>MSLGQQQVTLFWSGAITGPTSDAGAPYGAAVEDYCKWANERKLVPGVVFNCVVRDDQYNNANTQRFFEEAVDRFKIPVFLSYATGANLQLKPLIQELRIPTIPASMHIELIDPPNNDYIFLPTTSYSEQVVALLEYIAREKKGAKVALVVHPSPFGRAPVEDARKAARELGLQIVDVQEVGSGNLDNTALLKRFEQAGVEYVVHQNVAGPVANILKDAKRLGLKMRHLGAHYTGGPDLIALAGDAAEGFLWATSFYMAHEDTPGIRLQKEIGRKYGRPENFIESVNYTNGMLAAAIAVEAIRRAQERFKRITNETVYQAIVGMNGPNAFKPGFAVSTKQGVEIDFTKSEHTGA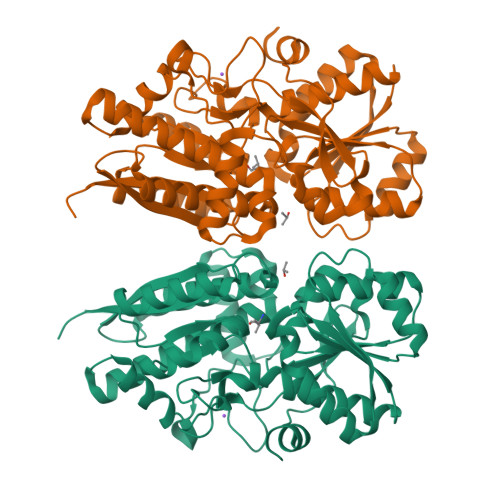EGLRILEAKGGRFVPVTEPFTSALFRKVHYGEGHHHHHH[2x]>GPLGS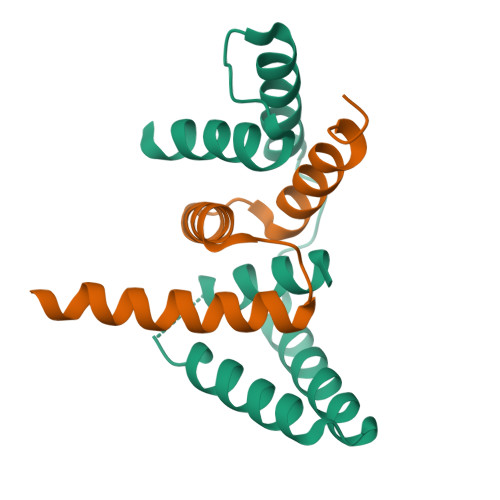MARHGPPWSRLDAQQERDVRELVRGVAGLQDEADPNFQLALNFAWSNFRFHRFLDVNSHKIEKTIEGIYEKFVIHSDLSKAASWKRLTEEFLNAPLPSIKEIKTDAHYSILSLLLCLSD[2x];>GPHMASSGGAGAAAAAAAANLNAVRETMDVLLEISRILNTGLDMETLSICVRLCEQGINPEALSSVIKELRKATEALKAAENMTS[2x]(2~{S})-2-acetamido-3-(4-hydroxyphenyl)-~{N}-prop-2-enyl-propanamide 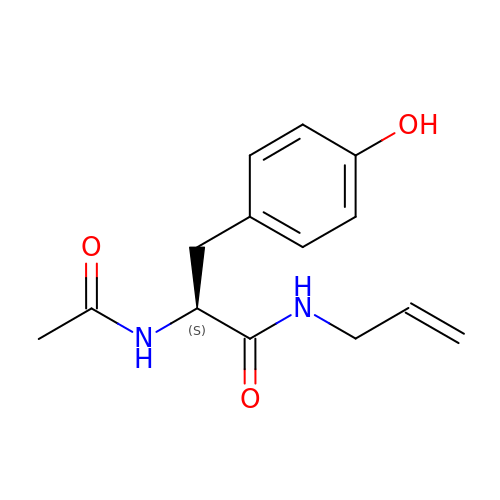| C14 H18 N2 O3 | OVAVZWLRPFXTJT-ZDUSSCGKSA-N5-[3,3-dimethyl-2-[5-(1,3,3-trimethylindol-2-ylidene)penta-1,3-dienyl]indol-1-ium-1-yl]-~{N}-[8-[[(1~{R},2~{S},3~{S},4~{S},5~{R})-2,3,4,5-tetrakis(oxidanyl)cyclohexyl]amino]octyl]pentanamide 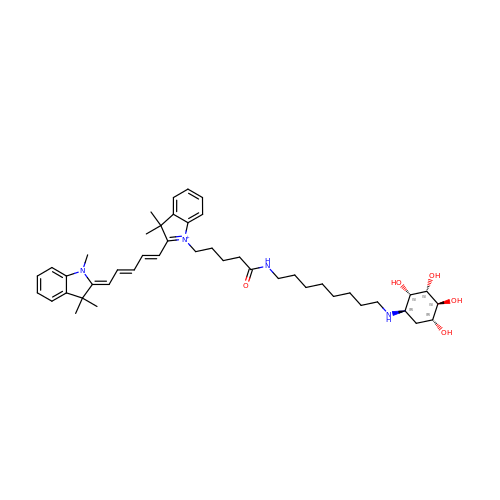| C45 H65 N4 O5 | QVZIJCUKVKFUJR-XDYJFVOXSA-O>[2x]SNAM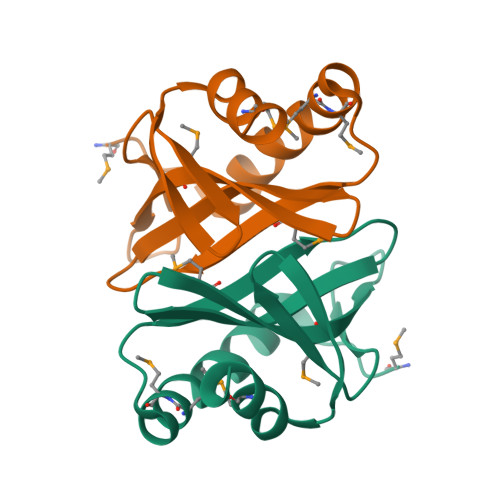EFAPRSVVIEEFIDTLEPMMEAYGLDQVGIFEEHGEGNRYYVGYTINKDDEMITIHMPFVKNERGELALEKQEWTVRKDGREKKGFHSLQEAMEEVIHS> MWGKVVVIGSGEYGKRAAQRVADLLDPRIDVYLIFDAKSTDEIRKMIKDHGADAV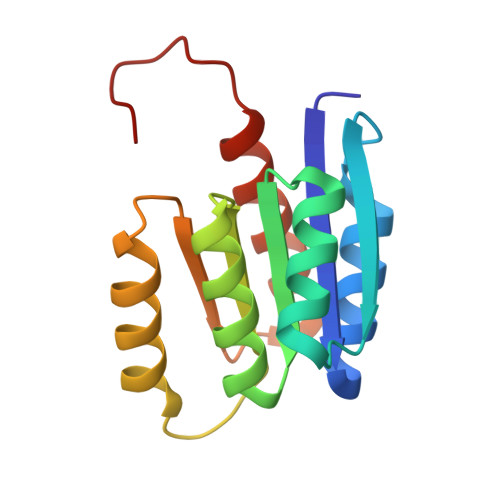IVIGAPLGTAFAIAKAAAELGAAVIVIIPRRPGVREAARRFGEEARKYGGRVEVLLGATVEEAVAFARRVVQQFFALEHHHHHH> MKDLVDTTAMYLRTIYELEEEGVTPLRARIAERLEQSGPTVSQTVAR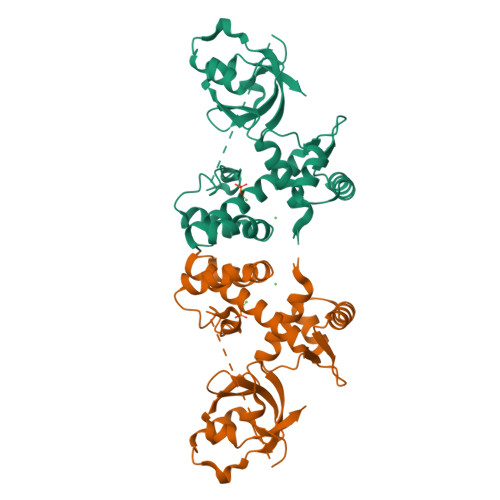MERDGLVVVASDRSLQMTPTGRTLATAVMRKHRLAERLLTDIIGLDINKVHDEADRWEHVMSDEVERRLVKVLKDVSRSPFGNPIPGLDELGVGNSDAAAPGTRVIDAATSMPRKVRIVQINEIFQVETDQFTQLLDADIRVGSEVEIVDRDGHITLSHNGKDVELLDDLAHTIRIEEL> GYCGPCPNNW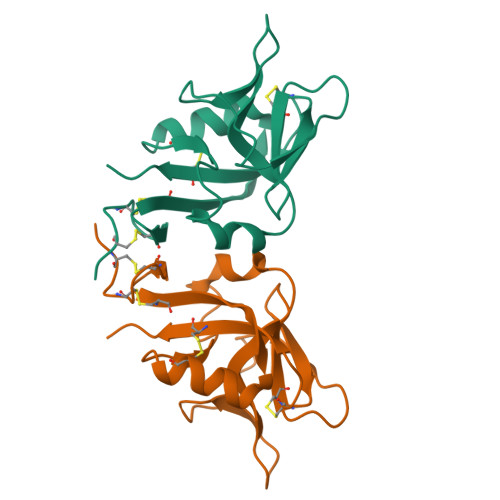ICHRNNCYQFFNEEKTWNQSQASCLSQNSSLLKIYSKEEQDFLKLVKSYHWMGLVQIPANGSWQWEDGSSLSYNQLTLVEIPKGSCAVYGSSFKAYTEDCANLNTYICMKRAV N-(1H-benzimidazol-2-yl)-1,3-dimethyl-1H-pyrazole-4-carboxamide | C13 H13 N5 O | 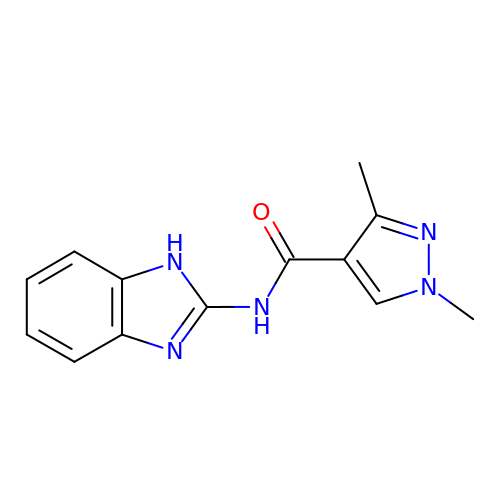ATWRDFSNOOXDOA-UHFFFAOYSA-N>MTSVTSKQSTILGSDEIDLGRVIGELIDHRKLIISITSVFTLFAILYALLATPIYETDALIQIEQKQGNAILSSLSQVLPDGQPQSAPETALLQSRMILGKTIDDLNLQIQIEQKYFPVIGRGLARLMGEKPGNIDITRLYLPDSDDISNNTPSIILTVKDKENYSINSDGIQLNGVVGTLLNEKGISLLVNEIDAKPGDQFVITQLPRLKAISDLLKSFSVADLGKDTGMLTLTLTGDNPKRISHILDSISQNYLAQNIARQAAQDAKS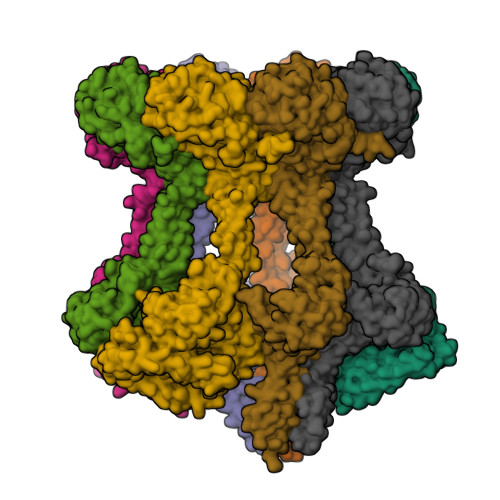LEFLNQQLPKVRAELDSAEDKLNAYRKQKDSVDLNMEAKSVLDQIVNVDNQLNELTFREAEVSQLYTKEHPTYKALMEKRQTLQEEKSKLNKRVSSMPSTQQEVLRLSRDVESGRAVYLQLLNRQQELNIAKSSAIGNVRIIDNAVTDPNPVRPKKTIIIVIGVVLGLIVSVVLVLFQVFLRRGIESPEQLEEIGINVYASIPISEWLTKNARQSGKVRKNQSDTLLAVGNPADLAVEAIRGLRTSLHFAMMEAKNNVLMISGASPSAGMTFISSNLAATIAITGKKVLFIDADLRKGYAHKMFGHKNDKGLSEFLSGQAAAEMIIDKVEGGGFDYIGRGQIPPNPAELLMHPRFEQLLNWASQNYDLIIIDTPPILAVTDAAIIGRYAGTCLLVARFEKNTVKEIDVSMKRFEQSGVVVKGCILNGVVKKASSYYRYGHNHYGYSYYDKKHHHHHH[8x]The GSR is a gene expression program that enables bacteria to cope with a range of adverse conditions such as oxidative stress, heat shock, and UV exposure. This response works using a so-called “partner-switching” mechanism, whereby HK activity—and subsequent phosphorylation of a downstream PhyR regulator —controls the activity of a transcriptional inhibitor known as NepR. Stress activates an HWE/HisKA2 HK, phosphorylating the PhyR and promoting sequestration of NepR away from σEcfG, allowing transcription of stress-responsive genes to occur. Exploring downstream effects of RT-HK, we identified two homologs of PhyR in the genome, RT-PhyR and RT-PhyR′. In the structures of both RT-PhyR and RT-PhyR′, we observed a typical arrangement between the SL and REC domains.

RT-PhyR and RT-PhyR′ were solved as a crystallographic trimer and a tetramer, respectively. Unsurprisingly, no electron density was present for the disordered loop in RT-PhyR′. Aligning the two PhyR paralog structures shows a reasonably high degree of overall similarity (2.7 Å Cα RMSD), with a notable major shift in the position of the loop connecting the β3 strand (immediately following the phosphoacceptor aspartate) and subsequent α10 helix (α3 in standard REC nomenclature). Adding other PhyR structures into the alignment (left), it is evident that RT-PhyR′ adopts an unusual conformation not routinely seen in other REC domains. This large-scale shift in RT-PhyR′ is likely related to the unique position of a conserved Q residue (Q193), which “leans in” and diminishes the solvent accessibility of the phosphoacceptor D (D191) (right). Two residues in the α9 helix of RT-PhyR′ also adopt distinct positions: a well-conserved R at the N terminus (R173) and another R at the C terminus (R184) “reach out” toward the typical position of the β3 loop and α10 helix, respectively. Notably, RT-PhyR′ was phosphorylated only at the longer timepoint and without a marked illumination dependence, suggesting that it is a nonspecific partner. On the other hand, addition of BeF3- to RT-NepR′-equilibrated RT-PhyR′ did not cause any substantial spectral shifts, showing that RT-PhyR′ binds RT-NepR′ to the exclusion of BeF3- rather than cooperatively. However, the analogous interactions seem to be inverted in RT-PhyR′, which exclusively binds RT-NepR′ when provided with both RT-NepR′ and BeF3-, suggesting a negatively cooperative function for this homolog. In contrast, the absence of a conformation representing the final inhibitory RT-PhyR′∼P/RT-NepR′ complex strongly suggests a phosphorylation-independent function for this homolog, the details of which remain unclear.

>GEFMPQTFADAVAASLPHLRRYARALTGEQRTGDAIAARTLEGLIADPSVLERDLEPRLMLFRAFHRTWRREGAPVGEADSHLAQRAQSHLARLTPNTREALLLHAIEGFTAQEIGAVMEVPPETAADFIDTALREMAESVAGRVMIIEDEAIIAMDIAAIVREMGHRVTGIARTRFEAVRLAREERPDLILADIQLADNSSGIDAVNEILAEFADLPVIFITAFPERLLTGERPEPAFLITKPYREEQVRSAVSQAMFFASTETLAA[4x]> MAGLLSTFDTFSSRRSESINKSGGGAVIPGQRSTVSVFVLGPSVTDDADKLSIATTFLAHSLDTDKQHSQRGGFLVSLLAMAYSSPELYLTTNGVNADVKYV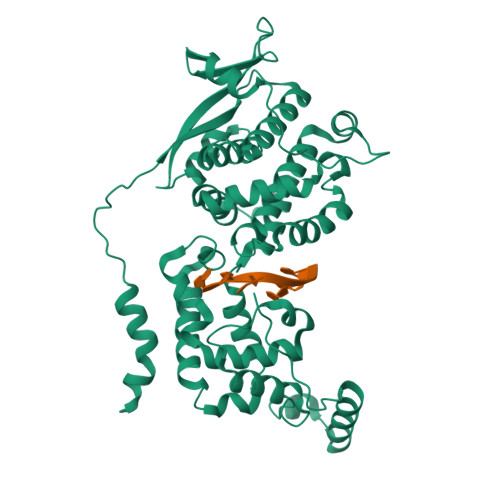IYNIEKDPKRTKTDGFIVKTRDMEYERTTEWLFGPMVNKSPLFQGQRDAADPDTLLQIYGYPACLGAIIVQVWIVLVKAITSSAGLRKGFFNRLEAFRQDGTVKGALVFTGETVEGIGSVMRSQQSLVSLMVETLVTMNTARSDLTTLEKNIQIVGNYIRDAGLASFMNTIKYGVETKMAALTLSNLRPDINKLRSLIDTYLSKGPRAPFICILKDPVHGEFAPGNYPALWSYAMGVAVVQNKAMQQYVTGRTYLDMEMFLLGQAVAKDAESKISSALEDELGVTDTAKERLRHHLANLSGGDGAYHKPTGGGAIEVALDNADIDLEPEAHTDQDARGWGGDSGDRWARSMGSGHFITLHGAERLEEETNDEDVSDIERRIARRLAERRQEDATTHEDEGRNNGVDHDEEDDAAAAAGMGGI> ALFDRLGRVVRANLNDLVSKAEDPEKVLEQAVIDMQEDLVQLRQAVARTIAEEKRTEQRLNQDTQEAKKWEDRAKLALTNGEENLAREALAR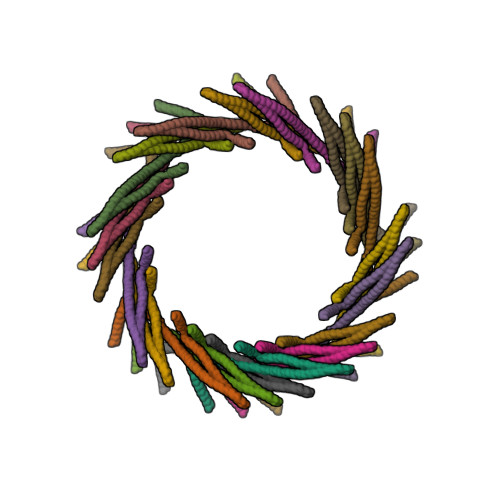KKSLTDTAAAYQTQLAQQRTMSENLRRNLAALEAKISEAKTKKNMLQARAKAAKANAELQQTLGGLGTSSATSAFERMENKVLDMEATSQAAGELAGFGIENQFAQLEASSGVEDELAALKAS> METRDQVKKLQLMLRQANDQLEKTMKDKQELEDFIKQSSEDSSHQISALVLRAQASEILLEELQQGLSQAKRDVQE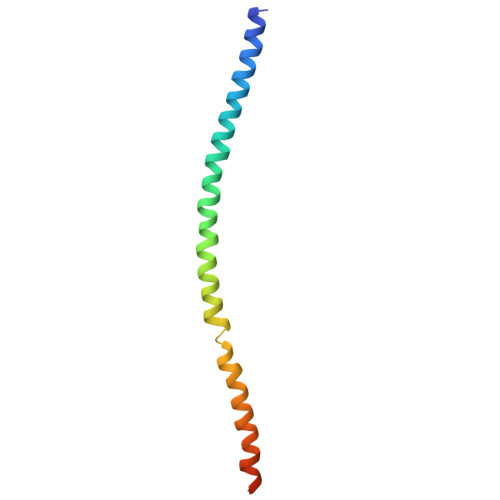QMAVLMQSREQVSEEL>[21x]MSFDNYLVPTVIEQSGRGERAFDIYSRLLKERIVFLVGPVTDESANLVVAQLL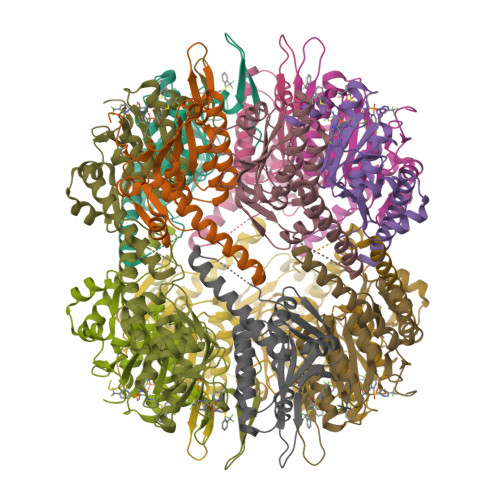FLESENPDKDIFFYINSPGGSVTAGMSIYDTMNFIKPDVSTLCLGQAASMGAFLLSAGEKGKRFALPNSRIMIHQPLISGGLGGQASDIEIHARELLKIKEKLNRLMAKHCDRDLADLERDTDRDNFMSAEEAKEYGLIDQILENRASLRL> SNARRGPAGIGRTGRGMGGLFSVGETTAKVLKDEIDVKFKDVAGCEEAKLEIMEFVNFLKNPKQYQDLGAKIPKGAILTGPPGTGKTLLAKATAGEANVPFITVSGSEFLEMFVGVGPARVRDLFALARKNAPCILFIDQIDAVGRKRGRGNFGGQSEQENTLNQLLVEMDGFNTTTNVVILAGTNRPDILDPALLRPGRFD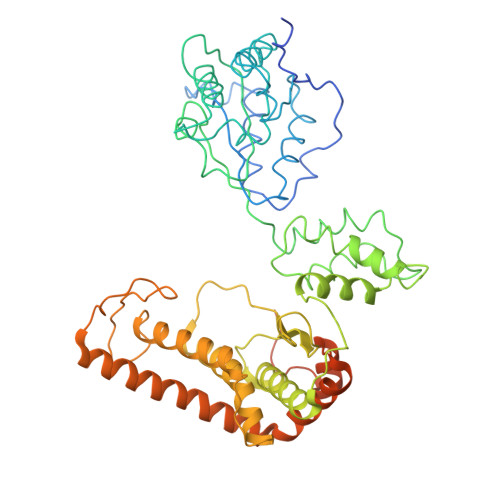RQIFIGPPDIKGRASIFKVHLRPLKLDSTLEKDKLARKLASLTPGFSGADVANVCNEAALIAARHLSDSINQKHFEQAIERVIGGLEKKTQVLQPEEKKTVAYHQAGHAVAGWYLEHADPLLKVSIIPRGKGLGYAQYLPKEQYLYTKEQLLDRMCMTLGGRVSEEIFFGRITTGAQDDLRKVTQSAYAQIVQFGMNEKVGQISFDLPRQGDMVLEKPYSEATARLIDDEVRILINDAYKRTVALLTEKKADVEKVALLLLEKEVLDKNDMVELLGPRPFAEKSTYEEFVEGTGSLDEDTSLPEGLKDWNKEREKEKEEPPGEKVAN>MSSKSDDFGSIVASGVTGSGDGNGNGNDWVEKAKDVLQTSVDAVTETAKKTKDVSDEMIPHVQQFLDSNPYLKDVIVPVSLTMTGTLFAWVVMPRILRRFHTYAMQSSAKLLPVGFSNEDVPYEKSFWGALEDPARYLVTFIAFAQIAAMVAPTTIAAQYFSPTVKGAVILSLVWFLYRWKTNVITRMLSAKSFGGLDREKVLTLDKVSSVGLFAIGLMASAEACGVAVQSILTVGGVGGVVTAFAARDILGNVLSGLSMQFSRPFSMGDTIKAGSVEGQVIEMGLTTTSLLNAEKFPVLVPNSLFSSQVIVNKSRAQWRAIASKIPLQIDDLDMIPQISNEIKEMLRSNTKVFLGKEAPHCYLSRVEKSFAELTIGCNLIRMGKEELYNTQQEVLLEAVKIIKKHGV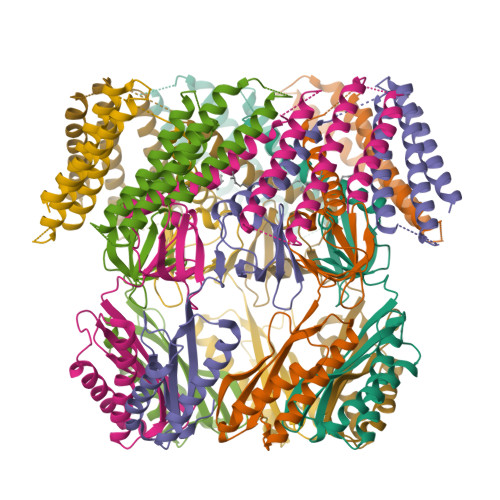SLGTTWDNSTLSNSLEVLFQ[7x]>TPEFGGNLQKVLVDLIELSLQGKQAHWNVVGSNFRDLHL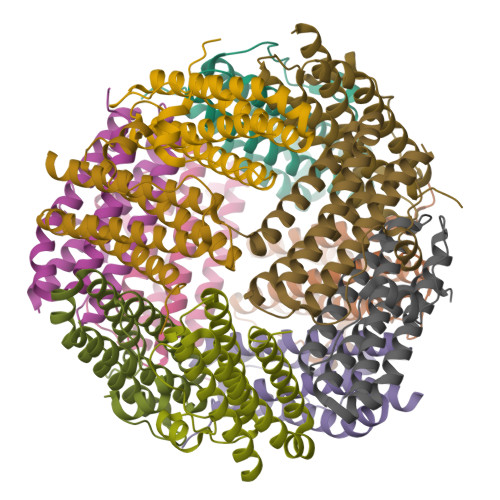QLDELVDFAREGSDTIAERMRALDAVPDGRSDTVAATTTLPEFPAFERSTADVVDLITTRINATVDTIRRVHDAVDAEDPSTADLLHGLIDGLEKQAWLIRSENRKV[12x]4-[(3R,3aS,6R,6aS)-6-(3-methoxy-4-oxidanyl-phenyl)-1,3,3a,4,6,6a-hexahydrofuro[3,4-c]furan-3-yl]-2-methoxy-phenol 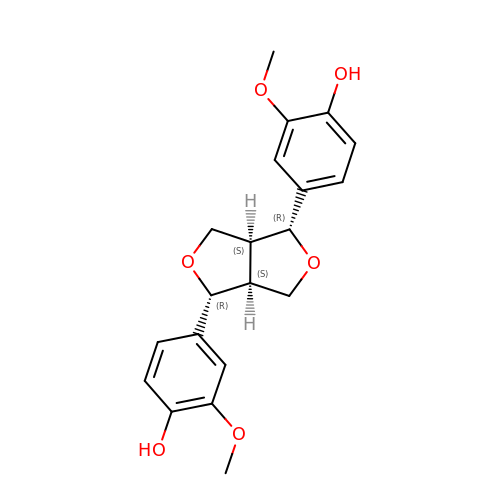| C20 H22 O6 | HGXBRUKMWQGOIE-NSMLZSOPSA-N> MARTGAEYIEALKTRPPNLWYKGEKVEDPTTHPVFRGIVRTMAALYDLQHDPRYREVLTYEEEGKRHGMSFLIPKTKEDLKRRGQAYKLWADQNLGMMGRSPDYLNAVVMAYAASADYFGEFAENVRNYYRYLRDQDLATTHALTNPQVNRARPPSGQPDPYIPVGVVKQTEKGIVVRGARMTATFPLADEVLIFPSTLLQAGSEKYALAFALPTSTPGLHFVCREALVGGDSPFDHPLSSRVEEMDCLVIFDDVLVPWERVFILGNVELCNNAYAATGALNHMAHQVVALKTAKTEAFLGVAALMAEGIGADVYGHVQEKIAEIIVYLEAMRAFWTRAEEEAKENAYGLLVPDRGALDGARNLYPRLYPRIREILEQIGASGLITLPSEKDFKGPLGPF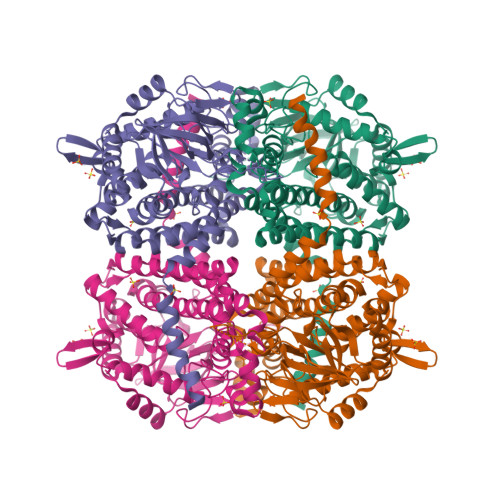LEKFLQGAALEAKERVALFRLAWDMTLSGFGARQELYERFFFGDPVRMYQTLYNVYNKEPYKERIRAFLKESLKVFEEVQA The (−)RNA genome of these viruses is condensed by a viral nucleoprotein (N) into a helical nucleocapsid, that associates with the polymerase complex and serves as the template for RNA replication and transcription. For non-segmented (−)RNA viruses of the Rhabdoviridae and Paramyxoviridae, N is assisted by the viral phosphoprotein (P). P binds to nascent RNA-free N, forming a N0-P complex (the superscript 0 denotes the absence of RNA) that prevents the polymerization of N and the non-specific encapsidation of host cell RNAs. These processes are independent of each other and, therefore, P has to fulfill two chaperone activities; blocking both RNA binding and self-assembly of N. P is a modular protein comprising a long N-terminal disordered region and two folded domains, a central oligomerization domain and a C-terminal nucleocapsid-binding domain, separated by a flexible linker.

In this study, we report the reconstitution of complexes between a recombinant N of VSV lacking the 21 N-terminal residues, NΔ21, and either full-length P dimer or a peptide encompassing the N0-binding MoRE of P, named here P60, that comprises the first 60 amino acids of P, a two-amino acid linker and a C-terminal His6-tag. The structure was solved at a resolution of 3.0 Å by molecular replacement using the structure of an N protomer derived from the N-RNA complex. The complex contained no RNA, but instead, in each protomer, residues 6 to 35 of P60 were visible in a groove formed by residues of the hinge region of N (aa 200–300) at the junction between NNTD and NCTD. Upon binding to NΔ21, the second fluctuating helix is stabilized and extends from amino acids 17 to 31. The MoRE of VSV P (aa 6–35) binds to the central hinge region of N mainly through hydrophobic interactions. The amphipathic α-helix of P, together with residues 14 to 16, inserts into a hydrophobic groove of N. Tyr14 perfectly fits into a small hydrophobic pocket. In addition, the complex is stabilized by three intermolecular salt bridges. Concomitantly, the other extremity of the MoRE (aa 6–13) docks in a shallow groove on the backside of the N protomer which, in the multimeric N-RNA complex, is occupied by the NNT-arm of the adjacent Ni−1 protomer and whose bottom is made up of the NCT-loop of the Ni+1 protomer. N, the N-terminal part of the MoRE of P will compete with the NNT-arm of a neighboring N molecule and therefore interferes with the polymerization of N in the absence of RNA. 0-P60 complex, the negative pole of P localizes in the RNA binding groove, while the positive pole docks on the backside of NCTD, modifying the distribution of electrostatic potentials on these surfaces of N and suggesting that electrostatics could play a role in orientating P before binding.

>GAMEDPVEYPADYFRKSKEIPLYINTTKSLSDLRGYVYQGLKSGNVSIIHVNSYLYGALKDIRGKLDKDWSSFGINIGKAGDTIGIFDLVSLKALDGVLPDGVSDASRTSADDKWLPLYLLGLYRVGRTQMPEYRKKLMDGLTNQCKMINEQFEPLVPEGRDIFDVWGNDSNYTKIVAAVDMFFHMFKKHECASFRYGTIVSRFKDCAALATFGHLCKITGMSTEDVTTWILNREVADEMVQMMLPGQEIDKADSYMPYLIDFGLSSKSPYSSVKNPAFHFWGQLTALLLRSTRARNARQPDDIEYTSLTTAGLLYAYAVGSSADLAQQFCVGDNKYTPDDSTGGLTTNAPPQGRDVVEWLGWFEDQNRKPTPDMMQYAKRAVMSLQGLREKTIGKYAKSEFDK[5x];>[5x]MDNLTKVREYLKSYSRLDQAVGEIDEIEAQRAEKSNYELFQEDGVEEHTKPSYFQAADDSLEHHHHHH>[8x]GARVAIVMGSKSDWATMQFAAEIFEILNVPHHVEVVSAHRTPDKLFSFAESAEEN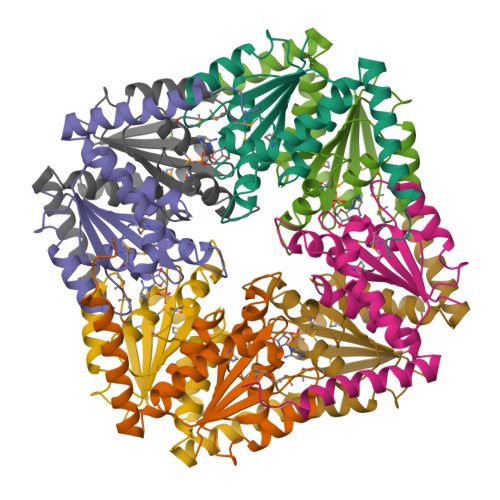GYQVIIAGAGGAAHLPGMIAAKTLVPVLGVPVQSAALSGVDSLYSIVQMPRGIPVGTLAIGKAGAANAALLAAQILATHDKELHQRLNDWRKAQTDEVLENPDPRG~{N}-[5-[(5-propan-2-yl-1,3-oxazol-2-yl)methylsulfanyl]-1,3-thiazol-2-yl]piperidine-4-carboxamide 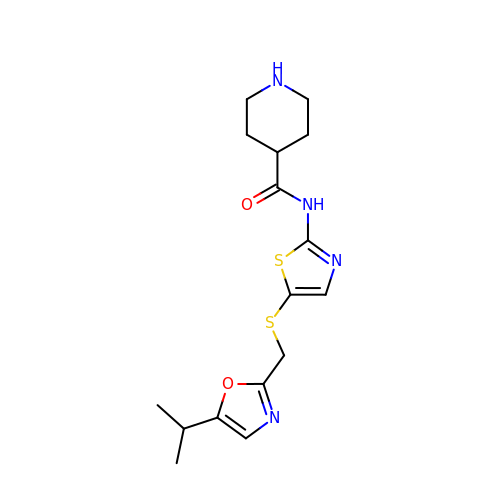| C16 H22 N4 O2 S2 | MCLDWKVRXDHDEI-UHFFFAOYSA-N>TTGGCCAA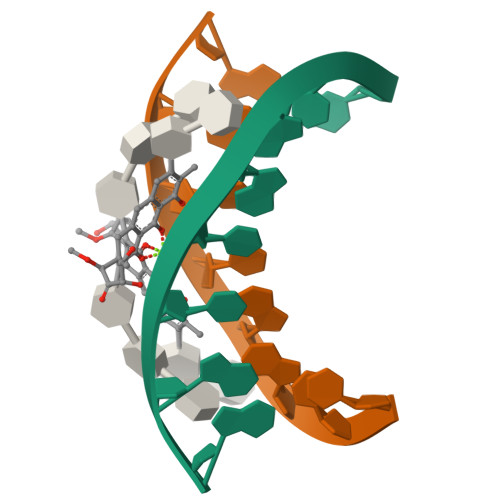[4x]[9-[2-carboxy-5-[2-[2-[4-(methylsulfonylamino)butoxy]ethoxy]ethylcarbamoyl]phenyl]-6-(dimethylamino)xanthen-3-ylidene]-dimethyl-azanium | C34 H43 N4 O8 S 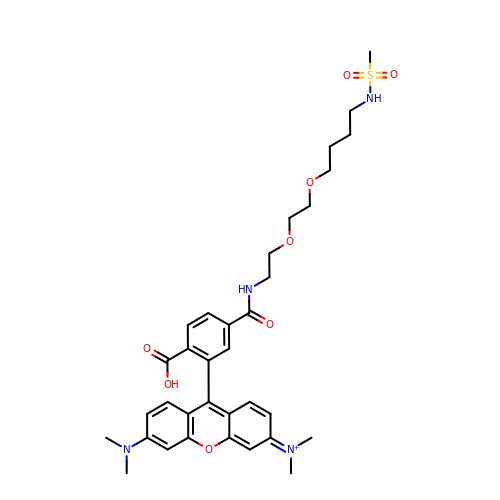| DSUCSFUEKBFNJW-UHFFFAOYSA-O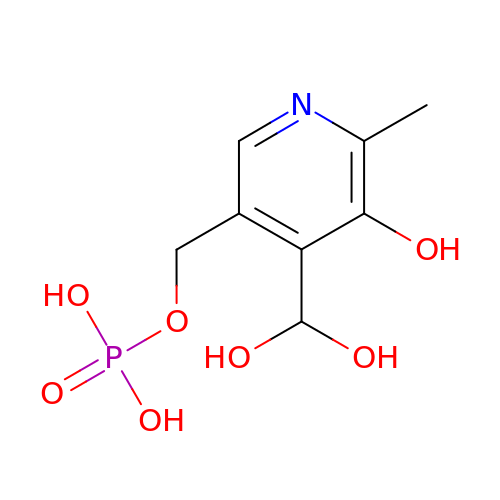[4-(DIHYDROXYMETHYL)-5-HYDROXY-6-METHYLPYRIDIN-3-YL]METHYL DIHYDROGEN PHOSPHATE | C8 H12 N O7 P | WNSLUVKENIMLGR-UHFFFAOYSA-N The tripartite motif (TRIM) proteins form one of the largest subfamilies of RING-type E3 ubiquitin ligases, comprising more than 80 members. TRIM family members typically contain a RING domain usually catalyzing ubiquitin transfer; one or two B-box domains mediating protein–protein interactions; and a large coiled-coil domain region, which is involved in self-association or oligomerization with other TRIM E3-ligase proteins (Fiorentini et al., 2020, Ozato et al., 2008). About two-thirds of human TRIM proteins feature a PRYSPRY domain, also known as the B30.2 domain, in their C-terminal region. All characterized family members shared the same overall PRYSPRY twisted β-sandwich fold consisting of a 7-stranded and a 6-stranded antiparallel β-sheet.

A characteristic feature of the putative substrate-binding site in the closely related homologs MID1 and MID2 is an arginine located at the C-terminus of β-strand 7 (R587 in MID1 and R637 in MID2) that projects its guanidinium group toward the center of the cavity and two neighboring tryptophan residues lining the pocket. MID1 is mutated in X-linked Opitz G/BBB syndrome, a rare genetic disorder that results in malformations along the midline of the body, including hypertelorism, hypospadias, and laryngo-tracheo-esophageal defects (Baldini et al., 2020, Trockenbacher et al., 2001). Many of the reported mutations map to the PRYSPRY domain (Baldini et al., 2020, Fontanella et al., 2008). Some of these, such as I536T and I555V, are large-to-small substitutions that potentially create internal cavities in the hydrophobic core of the β-sandwich, thereby reducing the thermodynamic stability of the domain. Like p53, the MID1 PRYSPRY domain is only moderately stable (DSF Tm of 47 °C), so it is also susceptible to global unfolding by cavity-creating mutations. The L626P mutation also perturbs the hydrophobic core of the β-sandwich and, being located in the middle of β-strand 11, also disrupts interstrand hydrogen bonds. The small-to-large mutation G532R introduces severe steric clashes and would bury a positive charge within a cluster of hydrophobic side chains, including Phe486 and Trp543. Therefore, this mutation is also likely to severely compromise the folding of the domain. The D611G mutation, for example, is located on the short loop connecting β-strands 9 and 10. This mutation results in the loss of a stabilizing hydrogen bond between the carboxylate group of Asp611 and the backbone nitrogen of Gly539 in the β3/β4 turn.

>[4x]SMNSQPFKLDPKSAHRKLKVSHDNLTVERDESSSKKSHTPERFTSQGSYGVAGNVFIDSGRHYWEVVISGSTWYAIGLAYKSAPKHEWIGKNSASWALCRCNNNWVVRHNSKEIPIEPAPHLRRVGILLDYDNGSIAFYDALNSIHLYTFDVAFAQPVCPTFTVWNKCLTIITGLPIPDHLDCTEQLP> MDSKYQCVKLNDGHFMPVLGFGTYAPAEVPKSKALEATKLAIEAGFRHIDSAHLYNNEEQVGLAIRSKIADGSVKREDIFYTSKLWCNSHRPELVRPALERSLKNLQLDYVDLYLIHFPVSVKPGEEVIPKDENGKILFDTVDLCATWEAVEKCKDAGLAKSIGVS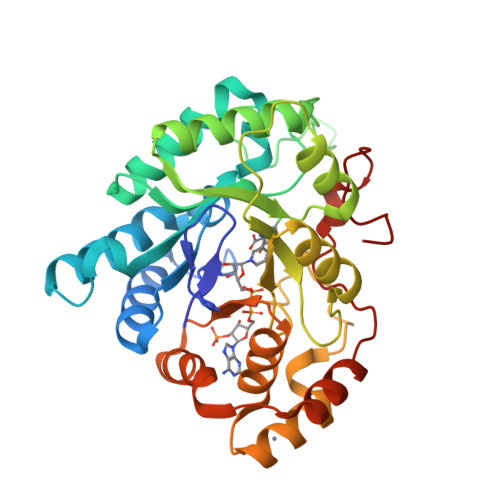NFNRRQLEMILNKPGLKYKPVCNQVECHPYFNQRKLLDFCKSKDIVLVAYSALGSHREEPWVDPNSPVLLEDPVLCALAKKHKRTPALIALRYQLQRGVVVLAKSYNEQRIRQNVQVFEFQLTSEEMKAIDGLNRNVRYLTVDIFAGPPNYPFSDEY>[3x]MIRIGHGFDVHAFGEDRPLIIGGVEVPYHTGFIAHSDGDVALHALTDAILGAAALGDIGKLFPDTDMQYKNADSRGLLREAFRQVQEKGYKIGNVDIT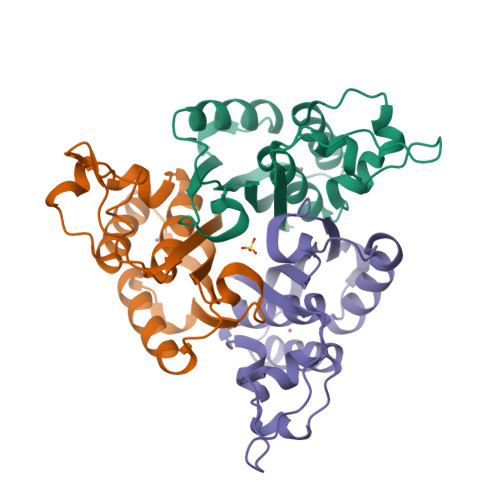IIAQAPKMRPHIDAMRAKIAEDLQCDIEQVNVKATTTEKLGFTGRQEGIACEAVALLIRQ> MGNSIKTLSNLANLLAQEG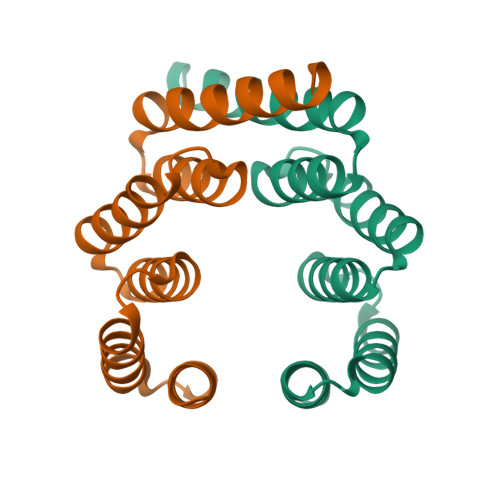KAEEAIKYMRKAVSLDPNNIKTLSNLANLLAQEGKAEEAIKYMRKAVSLDPNNIKTLSNLAVLLAQEGKAEEAIKYMRKAVSLIDKAAKG>[2x]MGLASLA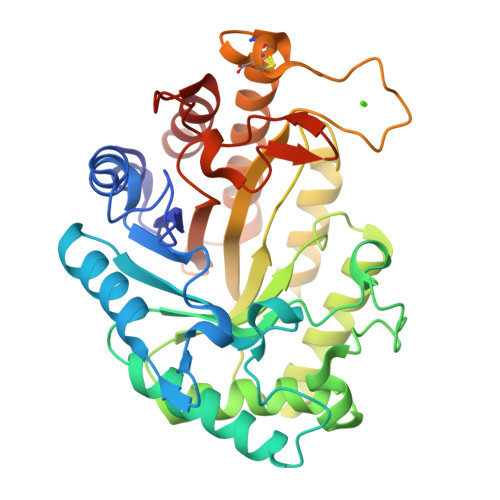DFPIGVAVAASGGNADIFTSSARQNIVRAEFNQITAENIMKMSYMYSGSNFSFTNSDRLVSWAAQNGQTVHGHALVWHPSYQLPNWASDSNANFRQDFARHIDTVAAHFAGQVKSWDVVNEALFDSADDPDGRGSANGYRQSVFYRQFGGPEYIDEAFRRARAADPTAELYYNDFNTEENGAKTTALVNLVQRLLNNGVPIDGVGFQMHVMNDYPSIANIRQAMQKIVALSPTLKIKITELDVRLNNPYDGNSSNDYTNRNDCAVSCAGLDRQKARYKEIVQAYLEVVPPGRRGGITVWGIADPDSWLYTHQNLPDWPLLFNDNLQPKPAYQGVVEALSGR>[2x]MSAHRTLLLRLSDSGEPVTSCSYGQGVLTLPSLPLPQGKKLGDMPVYTVKLAIPAGSPVTRDGLIWTNCPPDFSTQFDREKFYKKIIKTSFHEDDHIDLDIYVPGTYCFYLSFKNDKDELETTRKFYFVVLPILSVNDKFIPLNSIAMQSVVSKWMGPTIKDWEKVFARVASKKYNMIHFTPLQHRGESNSPYSIYDQLEFDPTVFKSEKEVADMVERLRTEHNILSLTDIVFNHTANNSQWLLDHPEAGYNHKTSPHLISAIELDKKLLDFSEQMEALGYPVDLKTVDDLIKVMDGIKEHVIGELKLWEFYVVDVKQTVSELREKWGNSKSWSDDNIPSKDDSTNLAQFVRDNATEPGFGSLGERGSNKINIDKFAAILKKLHSEDYNNGIEELATKILNDINLPFYKEYDDDINEVLEQLFNRIKYLRIDDHGPKQGPITKKLPLSEPYFTRFKAKDGEEYALANNGWIWDGNPLVDFASSQSKAYLRREVIVWGDCVKLRYGKGPSDSPYLWERMSKYVEMNARIFNGFRIDNCHSTPLHVGQYFLDVARRVNPNLYVVAQLFSGSEAMDCLFVERLGISSLIREAMQAWSEEELSRLVHRHGGRPIGSYKFVPLDDFPYPADVKIDEEYCAYNPDDHSVKCVSEIMIPKTLTATPPHALFMDCTHDNETPNQKRTVEDTLPNAALVAFCSSAIGSVYGYDEVFPQLL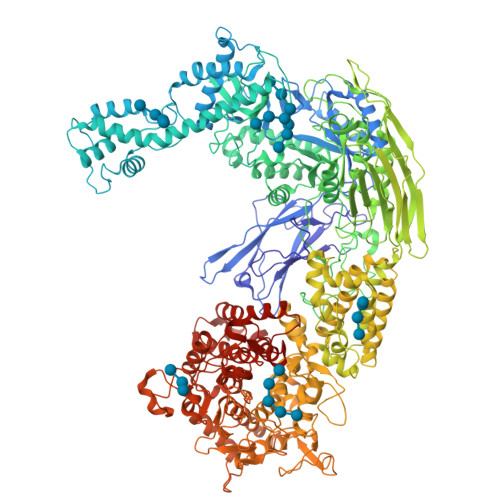DLVQEKRTYSCAENTGISKVKTLLNNMREEIASEAVDIEDSEMHVHHDGQYITFHRTNAKNGKGWYLVARTKFHSSGDQMLPRIKLSQTKATFKAAFSLERTGDAPISDEIIEGIPTKLRELTGFDIGFDENTKETSILLPQDFPQGSIVIFETQQLGIDDSLDHFIRSGAIKATEKLSLESINYVLYRAEQEEYDYSEGRSGAYDIPDYGKPVYCGLQGWVSILRKIIFYNDLAHPLSNNLRNGHWAVDYVVNRLDLYKDKEGVAEVQEWLRSRMERIKQLPSYLVPSFFALVVGIMYGCCRLRAMQLMSDNVGKSTVFVQSLAMTSIQMVSAMKSTSILPDQNIAAMAAGLPHFSTNYMRCWGRDVFISLRGLLLTTGRYEEAKEHILAFAKTLKHGLIPNLLDAGRNPRYNARDAAWFFVQAIQDYVTIVPGGVSLLQEKVTRRFPLDDEYIPYDDPKAFSYSSTIEEIIYEILNRHAGGIKYREANAGPNLDRVMKDEGFNVEVNVDWETGLIHGGSQFNCGTWMDKMGESEKANSVGVPGTPRDGAAVEINGLLKSCLRFVLQLSKDGKFKYTEVTKPDGSKISLSSWNDLLQENFERCFYVPKNKEDDNKFEIDATIINRRGIYKDLYRSGKPYEDYQFRPNFTIAMVVAPELFTPDYAAGAIELADQVLRGPVGMRTLDPSDYNYRPYYNNGEDSDDFATSKGRNYHQGPEWVWCYGYFIRAYHYFNFLTNPKCQVEGSAKKLKPSSYLYRKLYSRLLKHREWIENSPWAGLAELTNKDGEVCNDSSPTQAWSTGCLLDLFYDLWISYEE7-[5-(aminomethyl)pyridin-3-yl]-4-methylquinolin-2-amine | C16 H16 N4 | 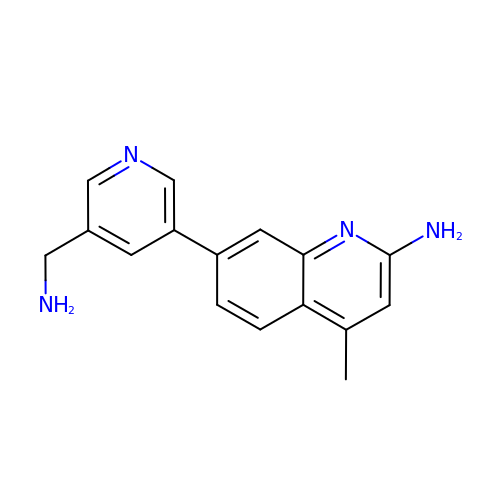HOBAPTQHAPAEBE-UHFFFAOYSA-N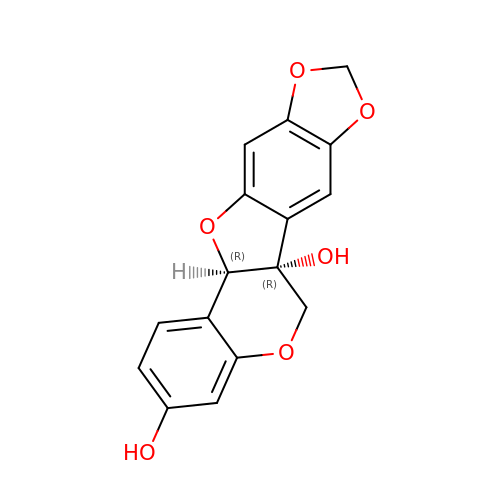(6AR,12AR)-6H-[1,3]DIOXOLO[5,6][1]BENZOFURO[3,2-C]CHROMENE-3,6A(12AH)-DIOL | C16 H12 O6 | GLMPLZUBQDAZEN-CVEARBPZSA-N> MVKYEDKISLYDAKGNLVEDGVPLEAISPLYNPTIKAMVKNIKRTVAVNLAGIENSLKTGAIGGKGCKVPGRTLDLPIVENAEAIMDEVEKILRITPDDDTQLRAINDGKQLVVQVPSKRLEVAAEYSVSMLNTAMALKEAIIKTF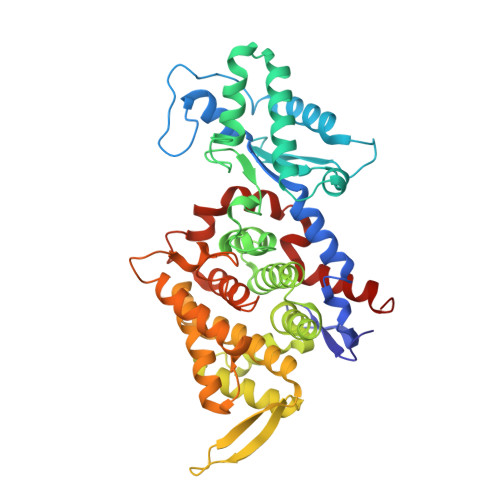DVDLFDGSTIHAAIVGRYPQVMDYMGGNIASLLGAPSNMEGLGYALRNIMVNHYVATTKKNLMNAVAFASIMEQTAMFEMGDAIGSFERMHLLGLAYQGLNSDNLVIDLVKANSKGTVGTVVASVVERALEDKVIVEDKSLESGFTMYKPADVAKWNAYAAAGLVAAVIVNCGAARAAQNVASTILYYNDILEYETGLPGTDFGRAEGTAVGFSFFSHSIYGGGGPGIFTGNHVVTRHSKGFAIPPVCAAMCADAGTQMFSPEKTSALVGAVYSAIDEFREPLKYVIEGALEVKDKI>[2x]MKITVLVGGVGGARFLLGVQNLLGLGSFADGPSKHELTAVVNIGDDAWMHGVRICPDLDTCMYTLGGGIDPDRGWGHRNETWNAKEELAAYGVQPDWFGLGDRDLATHLVRSQMLRAGYPLSQVTEALCKRWQPGARLLPASDERSETHVVITDPTDGERRAIHFQEWWVRYRAKVPTHSFAYVGADQATAGPGVVEAIGDADIVLLAPSNPVVSIGPILQIPGIRGALRSTSAPVIGYSPIIAGKPLRGMADECLKVIGVESTSQAVGEFFGARAGTGLLDGWLVHEGDHAQIEGVKVKAVPLLMTDPEATAAMVRAGLDLAGVSL

F420 is a low-potential redox cofactor used by diverse bacteria and archaea. In mycobacteria, this cofactor has multiple roles, including adaptation to redox stress, cell wall biosynthesis, and activation of the clinical antitubercular prodrugs pretomanid and delamanid. To determine the structural basis of dehydro-F420-0 production, we solved high-resolution crystal structures of the enzyme responsible (FbiA) in apo-, substrate-, and product-bound forms. The crystal structure of FbiA shows that this enzyme employs a flexible active site to capture Fo and EPPG, precisely positioning them for catalysis.

In order to resolve the catalytic mechanism of DH-F420-0 synthesis, purified FbiA was crystallized, and its structure was determined at 2.3 Å by X-ray crystallography. FbiA crystallized as a dimer mediated by the interaction of three α-helices and a β-sheet. This dimer is predicted to be stable by the protein-interaction prediction program PISA, and the molecular weight of FbiA determined by size exclusion chromatography coupled to multiangle light scattering (SEC-MALS) shows that it forms a dimer in solution. The structure of CofD from M. mazei, a homologous enzyme that instead utilizes LPPG derived from 2PL as its substrate, also crystallized as a dimer with an analogous interface to FbiA. The crystal structure of FbiA reveals an active site with open and closed states.>AMGNELPGTSDTPLLDQIHGPKDLKRLSREQLPALTEELRGEIVRVCSRGGLHLASSLGAVDIITALHYVLDSPRDRILFDVGHQAYAHKILTGRRDQMADIKKEGGISGFTKVSESEHDAITVGHASTSLANALGMALARDAQGKDFHVAAVIGDGSLTGGMALAALNTIGDMGRKMLIVLNDNEMSISENVGAMNKFMRGGGGGGGSVNPFAAMGVRYVGPVDGHNVQELVWLLERLVDLDGPTILHIVTTKGKGLSYAEADPIYWHGPAKFDP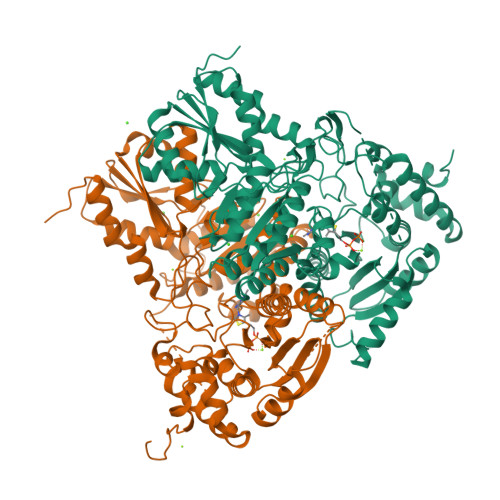ATGEYVPSSAYSWSAAFGEAVTEWAKTDPRTFVVTPAMREGSGLVEFSRVHPHRYLDVGIAEEVAVTTAAGMALQGMRPVVAIYSTFLQRAYDQVLHDVAIEHLNVTFCIDRAGIVGADGATHNGVFDLSFLRSIPGVRIGLPKDAAELRGMLKYAQTHDGPFAIRYPRGNTAQVPAGTWPDLKWGEWERLKGGDDVVILAGGKALDYALKAAEDLPGVGVVNARFVKPLDEEMLREVGGRARALITVEDNTVVGGFGGAVLEALNSMNLHPTVRVLGIPDEFQEHATAESVHARAGIDAPAIRTVLAELGVDVPIEV[2x]>[2x]TVPDNLKKQLAVSVRNIQWSYGIFWSVSASQPGVLEWGDGYYNGDIKTR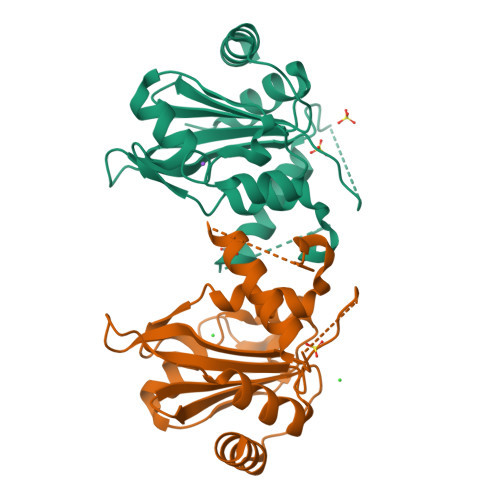KTIQAAEVKIDQLGLERSEQLRELYESLSLAESSASGSSQVTRRASAAALSPEDLTDTEWYYLVCMSFVFNIGEGIPGGALSNGEPIWLCNAETADSKVFTRSLLAKSASLQTVVCFPFLGGVLEIGTTEHIKEDMNVIQSVKTLFLEA>[2x]LPRPIRNLEVKFTKIFINNEWHESKSGKKFATCNPSTREQICEVEEGDKPDVDKAVEAAQVA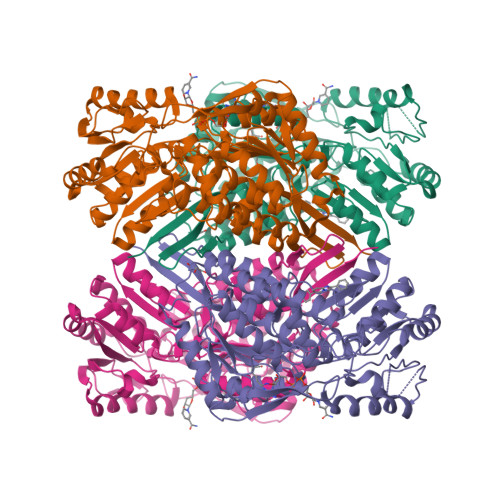FQRGSPWRRLDALSRGRLLHQLADLVERDRATLAALETMDTGKPFLHAFFIDLEGCIRTLRYFAGWADKIQGKTIPTDDNVVCFTRHEPIGVCGAITPWNFPLLMLVWKLAPALCCGNTMVLKPAEQTPLTALYLGSLIKEAGFPPGVVNIVPGFGPTVGAAISSHPQINKIAFTGSTEVGKLVKEAASRSNLKRVTLELGGKNPCIVCADADLDLAVECAHQGVFFNQGQCCTAASRVFVEEQVYSEFVRRSVEYAKKRPVGDPFDVKTEQGPQIDQKQFDKILELIESGKKEGAKLECGGSAMEDKGLFIKPTVFSEVTDNMRIAKEEIFGPVQPILKFKSIEEVIKRANSTDYGLTAAVFTKNLDKALKLASALESGTVWINCYNALYAQAPFGGFKMSGNGRELGEYALAEYTEVKTVTIKLG> MKFGNFLLTYQPPELSQTEVMKRLVNLGKASEGCGFDTVWLLEHHFTEFGLLGNPYVAAAHLLGATETLNVGTAAIVLPTAHPVRQAEDVNLLDQMSKGRFRFGICRGLYDKDFRVFGTDMDNSRALMDCWYDLMKEGFNEGYIAADNEHIKFPKIQLNPSAYTQGGAPVYVVAESASTTEWAAERGLPMILSWIINTHEKKAQLDLYNEVATEHGYDVTKIDHCLSYITSVDHDSNRAKDICRNFLGHWYDSYVNATKIFDDSDQTKGYDFNKGQWRDFVLKGHKDTNRRIDYSYEINPVGTPEECIAIIQQDIDATGIDNICCGFEANGSEEEIIASMKLFQSDVMPYLKEKQ;> MKFGLFFLNFMNSKRSSDQVIEEMLDTAHYVDQLKFDTLAVYENHFSNNGVVGAPLTVAGFLLGMTKNAKVASLNHVITTHHPVRVAEEACLLDQMSEGRF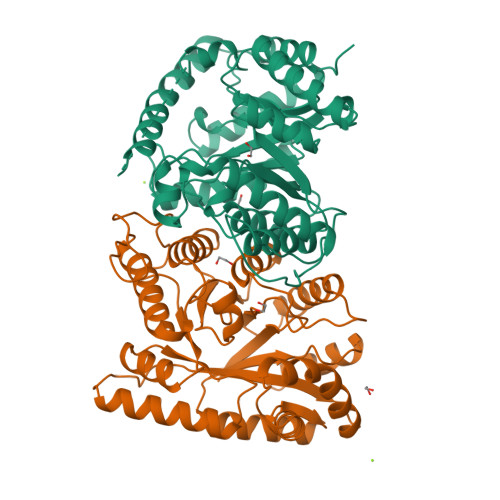AFGFSDCEKSADMRFFNRPTDSQFQLFSECHKIINDAFTTGYCHPNNDFYSFPKISVNPHAFTEGGPAQFVNATSKEVVEWAAKLGLPLVFRWDDSNAQRKEYAGLYHEVAQAHGVDVSQVRHKLTLLVNQNVDGEAARAEARVYLEEFVRESYSNTDFEQKMGELLSENAIGTYEESTQAARVAIECCGAADLLMSFESMEDKAQQRAVIDVVNANIVKYHS>SNAEKEKDTIAAEHKQEASVLLNLHRNKINYLIGETMARMTSLSIAIDRPVDIKKM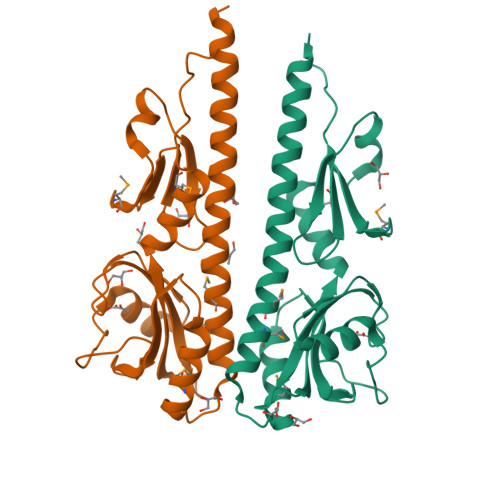QSILEKTFDSEPRFSGLYFLNAKGDVTASTTELKTKVNLADRSFFIKAKETKKTVISDSYSSRITGQPIFTICVPVLDSKRNVTDYLVAAIQIDYLKNLINLLSPDVYIEVVNQDGKMIFASGQASHAEDQKPVSGYLDDISWNMKVYPNPVTIEELSKSL[2x]> NVLPSELPAGVDWRSRGCVTPVKDQRDCGSCWAFSTTGALEGAHCAKTGKLVSLSEQELMDCSRAEGNQSCSGGEMNDAFQYVLDS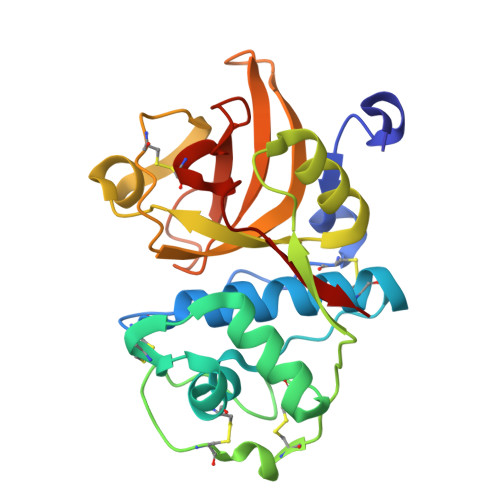GGICSEDAYPYLARDEECRAQSCEKVVKILGFKDVPRRSEAAMKAALAKSPVSIAIEADQMPFQFYHEGVFDASCGTDLDHGVLLVGYGTDKESKKDFWIMKNSWGTGWGRDGYMYMAMHKGEEGQCGLLLDASFPVM> VHITLDPDTANPWLILSEDRRQVRLGDTQQSIPGNEERFDSYPMVLGAQHFHSGKHYWEVDVTGKEAWDLGVCRDSVRRKGHFLLSSKSGFW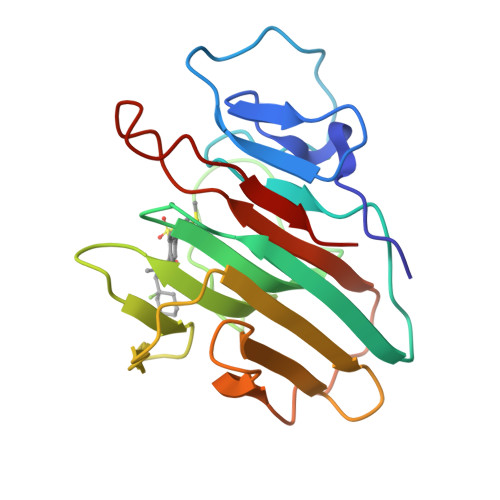TIWLWNKQKYEAGTYPQTPLHLQVPPCQVGIFLDYEAGMVSFYNITDHGSLIYSFSECAFTGPLRPFFSPGFNDGGKNTAPLTALC> MEH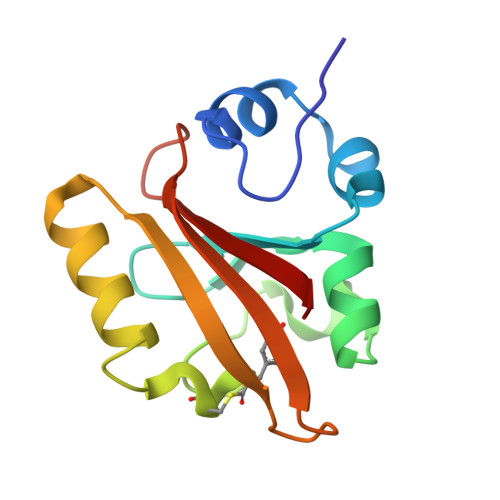VAFGSEDIENTLAKMDDGQLDGLAFGAIQLDGDGNILQYNAAEGDITGQDPKQVIGKNFFKDVAPCTDSPEFYGKFKEGVASGNLNTMFEYTFDYQMTPTKVKVHMKKALSGDSYWVFVKRV>MANLHALRREQRAQGPATIMAIGTATPPNLYEQSTFPDFYFRVTNSDDKQELKKKFRRMCEKTMVKKRYLHLTEEILKERPKLCSYKEASFDDRQDIVVEEIPRLAKEAAEKAIKEWGRPKSEITHLVFCSISGIDMPGADYRLATLLGLPLTVNRLMIYSQACHMGAAMLRIAKDLAENNRGARVLVVACEITVLSFRGPNEGDFEALAFQAGFGDGAGAVVVGADPLEGIEKPIYEIAAAMQETVAESQGAVGGHLRAFGWTFYFLNQLPAIIADNLGRSLERALAPLGVREWNDVFWVAHPGNWAIIDAIEAKLQLSPDKLSTARHVFTEYGNM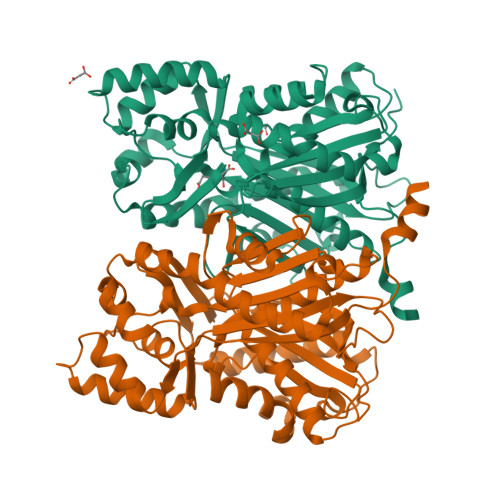QSATVYFVMDELRKRSAVEGRSTTGDGLQWGVLLGFGPGLSIETVVLRSMPLHHHH[4x]> MQTTVTTMLLASVALAACAGGGSTPLPLPQQQPPQQEPPPPPVPLASRAACEALKDGNGDMVWPNAATVVEVAAWRDAAPATASAAALPEHCEVSGAIAKRTGIDGYPYEIKFRLRMPAEWNGRFFMEGGS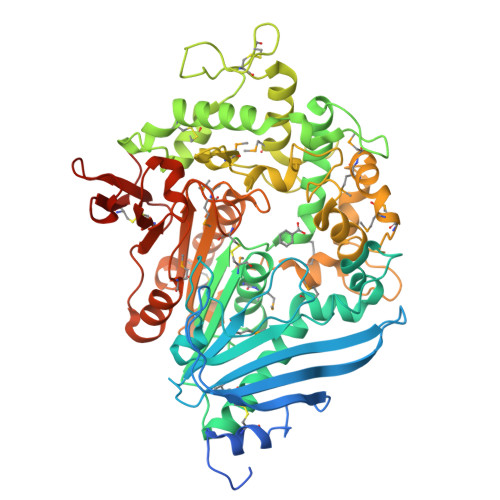GTNGSLSAATGSIGGGQIASALSRNFATIATDGGHDNAVNDNPDALGTVAFGLDPQARLDMGYNSYDQVTQAGKAAVARFYGRAADKSYFIGCSEGGREGMMLSQRFPSHYDGIVAGAPGYQLPKAGISGAWTTQSLAPAAVGLDAQGVPLINKSFSDADLHLLSQAILGTCDALDGLADGIVDNYRACQAAFDPATAANPANGQALQCVGAKTADCLSPVQVTAIKRAMAGPVNSAGTPLYNRWAWDAGMSGLSGTTYNQGWRSWWLGSFNSSANNAQRVSGFSARSWLVDFATPPEPMPMTQVAARMMKFDFDIDPLKIWATSGQFTQSSMDWHGATSTDLAAFRDRGGKMILYHGMSDAAFSALDTADYYERLGAAMPGAAGFARLFLVPGMNHCSGGPGTDRFDMLTPLVAWVERGEAPDQISAWSGTPGYFGVAARTRPLCPYPQIARYKGSGDINTEANFACAAPPLEHHHHHH Unlike most NLRs, the plant NLR required for cell death 2 (NRC2) belongs to a small NLR group characterized by constitutively high expression without self-activation. In this study, we discovered that SlNRC2 forms dimers and tetramers and higher-order oligomers at elevated concentrations. Using cryo-electron microscopy (cryo-EM), we performed structural analyses and found that SlNRC2 adopts an inactive conformation in both the dimeric and oligomeric states. Structural comparison shows that SlNRC2 dimerization and oligomerization act to stabilize the inactive conformation.

Electron microscopy negative-staining indicated that SlNRC2 from this peak contained filaments and aggregates. When concentrated, the SlNRC2 protein from the 200–300 kDa peak also formed filaments with similar morphology to those directly eluted from the void volume. Further analysis was then conducted on a subset of 611,661 particles for the dimer and 159,294 particles for the tetramer, resulting in a cryo-EM density map with resolutions of 2.84 and 3.17 Å, respectively. The cryo-EM structure of the filament was determined following the methods previously described. A total of 280,426 particles with more coherent helical parameters were used for the final 3D refinement process. The resulting cryo-EM reconstruction of the filament sample achieved an overall resolution of 3.6 Å. The SlNRC2 filament consists of three protofilaments. Only marginal contacts mediate the interprotofilament interactions. Both dimeric and tetrameric SlNRC2 structures are present in the filament. Each protofilament contains several copies of tetrameric SlNRC2. Filament propagation probably involves the incorporation of dimeric SlNRC2 into pre-existing filaments.

>[12x]MANVAVEFLVENLMQLLRDNVELISGVKEAAESLLQDLNDFNAFLKQAAKCHINENEVLRELVKKIRTVVNSAEDAIDKFVIEAKLHKDKGVTRVLDLPHYKRVKEVAGEIKAIRNKVREIRQTDAIGLQALQDDDLSARGSEERKPPVVEEDDVVGFDEEADIVINRLLGESNHLEVVPVVGMPGLGKTTLANKIYKHPKIGYEFFTRIWVYVSQSYRRRELFLNIISKFTRNTKQYHGMCEEDLADEIQEFLGKGGKYLVVLDDVWSDEAWERIKIAFPNNNKPNRVLLTTRDSKVAKQCNPIPHDLKFLTEDESWILLEKKVFHKDKCPPELVLSGKSIAKKCKGLPLAIVVIAGALIGKGKTPREWKQVDDSVSEHLINRDHPENCNKLVQMSYDRLPYDLKACFLYCSAFPGGFQIPAWKLIRLWIAEGFIQYKGHLSLECKGEDNLNDLINRNLVMVMERTSDGQIKTCRLHDMLHEFCRQEAMKEENLFQEIKLGSEQYFPGKRELSTYRRLCIHSSVLDFFSTKPSAEHVRSFLSFSSKKIEMPSADIPTIPKGFPLLRVLDVESINFSRFSREFYQLYHLRYVAFSSDSIKILPKLMGELWNIQTIIINTQQRTLDIQANIWNMERLRHLHTNSSAKLPVPVAPKNSKVTLVNQSLQTLSTIAPESCTEEVFARTPNLKKLGIRGKISVLLDNKSAASLKNVKRLEYLENLKLINDSSIQTSKLRLPPAYIFPTKLRKLTLLDTWLEWKDMSILGQLEHLEVLKMKENGFSGESWESTGGFCSLLVLWIERTNLVSWKASADDFPRLKHLVLICCDNLKEVPIALADIRSFQVMMLQNSTKTAAISARQIQAKKDNQTQQGTKNIAFKLSIFPPDL Kinesins are a superfamily of microtubule (MT)-based molecular motors that play important roles in cellular functions such as mitosis, cell motility, and intracellular transport. The kinesin motor domain is the MT-binding engine that drives these activities, converting the chemical energy of ATP binding and hydrolysis into mechanical force. Recently, it has been demonstrated that a subset of kinesin superfamily members, including kinesin-2s, −3 s, −8 s, and −12 s, are sequestered by kinesin-binding protein (KBP; KIF1BP; KIAA1279), which inhibits MT track attachment by their motor domains and, thus, blocks their MT-related functions. Here we present cryo-electron microscopy (cryo-EM) structures of KBP alone and of KBP bound to the motor domain of the human mitotic kinesin KIF15 (a 110 kDa complex).

The 3D structure of the ~72 kDa KBP at 4.6 Å resolution was determined using cryo-EM data collected using a Volta phase plate (VPP), and an atomic model was calculated. Our structure revealed that KBP is a right-handed α-solenoid protein. Nine pairs of anti-parallel α-helices (αHP1 [α-helical pair 1] to αHP9) are broken by a single ‘linker α-helix’ (LαH) and ‘linker loop’ (LL) in the centre of the fold separating KBP into N-terminal and C-terminal subdomains. The four predicted TPR motifs contribute exclusively to α-helical pairs in the N-terminal subdomain. The supercoiling α-helical pairs form concave and convex faces linked by short and long loops that constitute the two edges of the α-solenoid. In contrast to the shorter loops, the longer loops (more than seven residues) tend to be partially disordered, show low sequence homology between KBP orthologues in different species, and are mainly found in the N-terminal subdomain (e.g. L2, L6, and L10). The LL is the longest (62 residues) and is thus unique in the KBP structure because it is reasonably conserved and mainly ordered, with visible corresponding density clearly bridging the N- and C-terminal subdomains. Despite this clear ordered density, this loop was not modelled due to low homology to available structures and a lack of consensus in secondary structure prediction. In spite of this lack of consensus, density in this region suggests that part of this loop may form further α-helical structures. The KBP-alone model is incompatible with KIF15_MD6S binding, due to clashes with L14 in the C-terminal subdomain and αHP3a, αHP4a, and L8 in the N-terminal subdomain.

> MANVPWAEVCEKFQAALALSRVELHKNPEKEPYKSKYSARALLEEVKALLGPAPEDEDERPEAEDGPGAGDHALGLPAEVVEPEGPVAQRAVRLAVIEFHLGVNHIDTEELSAGEEHLVKCLRLLRRYRLSHDCISLCIQAQNNLGILWSEREEIETAQAYLESSEALYNQYMKEVGSPPLDPTERFLPEEEKLTEQERSKRFEKVYTHNLYYLAQVYQHLEMFEKAAHYCHSTLKRQLEHNAYHPIEWAINAATLSQFYINKLCFMEARHCLSAANVIFGQTGKISATEDTPEAEGEVPELYHQRKGEIARCWIKYCLTLMQNAQLSMQDNIGELDLDKQSELRALRKKELDEEESIRKKAVQFGTGELCDAISAVEEKVSYLRPLDFEEARELFLLGQHYVFEAKEFFQIDGYVTDHIEVVQDHSALFKVLAFFETDMERRCKMHKRRIAMLEPLTVDLNPQYYLLVNRQIQFEIAHAYYDMMDLKVAIADRLRDPDSHIVKKINNLNKSALKYYQLFLDSLRDPNKVFPEHIGEDVLRPAMLAKFRVARLYGKIITADPKKELENLATSLEHYKFIVDYCEKHPEAAQEIEVELELSKEMVSLLPTKMERFRTKMALT>[11x]MELIHPENGPSGTVQVPLIQGVDQSDTEDVYRLSPHVTTGFADTFKESNDIMGFSFMEKVNGAIYKYTHFAFY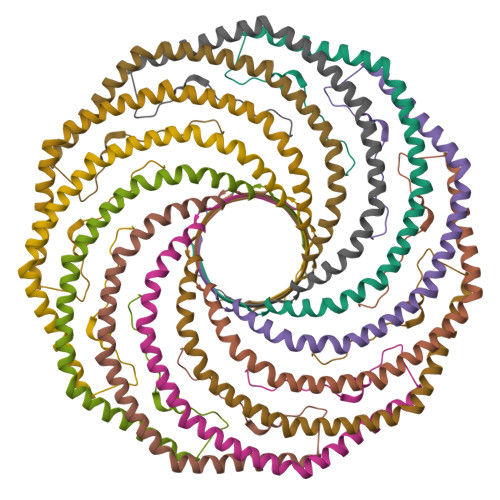AVLNLLLAPFIAFSFGLSFAVMHFAVVWFVQPIMKLYYVWLRVFNLAYEPALRLVCDPIHRSIALILSGIKGQFKMNSSDVKTSQV>[3x]MMFIVNTNVPRASVPDGFLSELTQQLAQATGKPPQYIAVHVV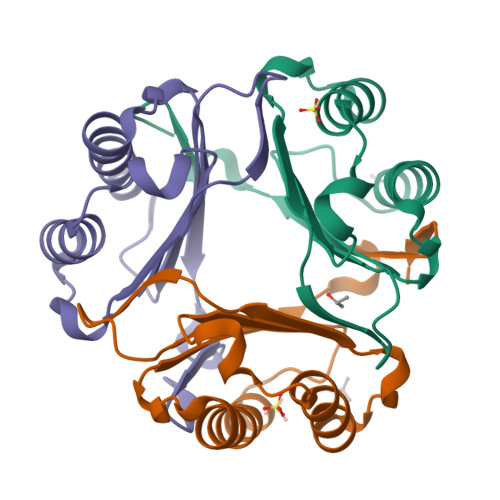PDQLMAFGGSSEPCALCSLHSIGKIGGAQNRSYSKLLCGLLAERLRISPDRVYINYYDMNAANVGWNNSTFA>MSSALLRAAYAYDRLRAHPPEVAGQIATAMASAVHPKGEEPVFLELGVGTGRIALPLIARGYRYIALDADAAMLEVFRQKIAGVDRKVQVVQADARAIPLPDESVHGVIVVHLWHLVPDWPKVLAEAIRVLKPGGALLEGWDQAEASPEWTLQ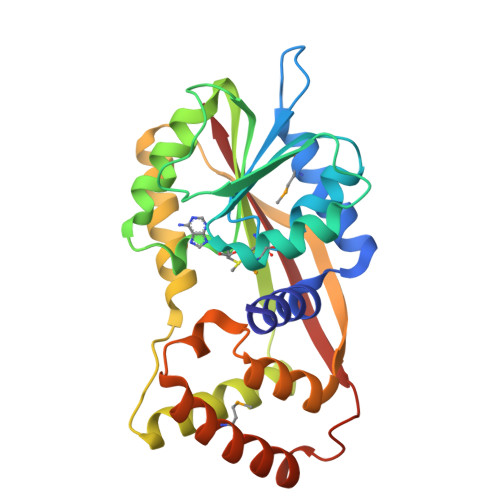ERWRAFAAEEGFPVERGLHAKRLKEVEEALRRLGLKPRTREVARWREERTPREALEALSERLYSFTQGLPEPVHARVMERLWAWAEAELGDLDRPFPVEKRFLLRVSRLG[2x]> ADVTIT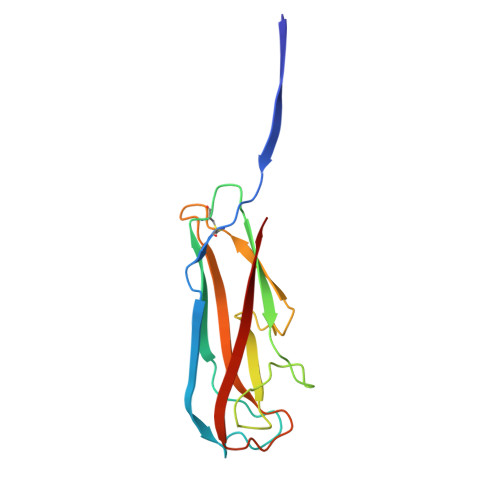VNGKVVAKPCTVSTTNATVDLGDLYSFSLMSAGAASAWHDVALELTNCPVGTSRVTASFSGAADSTGYYKNQGTAQNIQLELQDDSGNTLNTGATKTVQVDDSSQSAHFPLQVRALTVNGGATQGTIQAVISITYTYS> MFNAKYVAEATGNFITVMD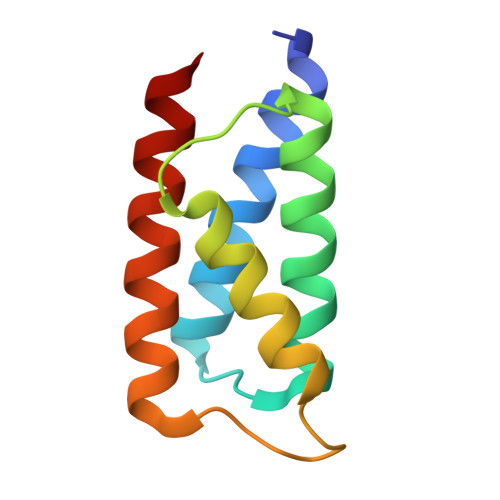ALKLNYNAKDQLHPLLAELLISINRVTRDDFENRSKLIDWIVRINKLSIGDTLTETQIRELLFDLELAYKSFYALLD> ALEHEKTPELAAKLAAEAIERDPWAAQVSQLSLPKLVEQVALNAWKEESDNAVCLHLRSSQRHLNNRGAQQKLAEALSMLKGSTVELTIVEDDNPAVRTPLEWRQAIYEEKL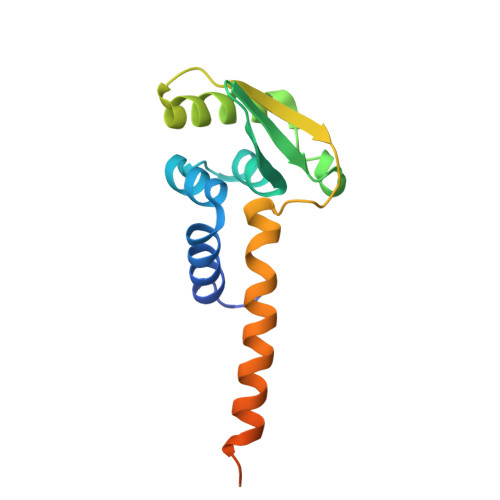AQARESIIADNNIQTLRRFFDAELDEESIRPI>MVLGKPQTDPTLEWFLSHCHIHKYPSKSTLIHQGEKAETLYYIVKGSVAVLIKDEEGKEMILSYLNQGDFIGELGLFEEGQERSAWVRAKTACEVAEISYKKFRQLIQVNPDILMRLSAQMARRLQVTSEKVGNLAFLLVTGRIAQTLLNLAKQPDAMTHPDGMQIKITRQEI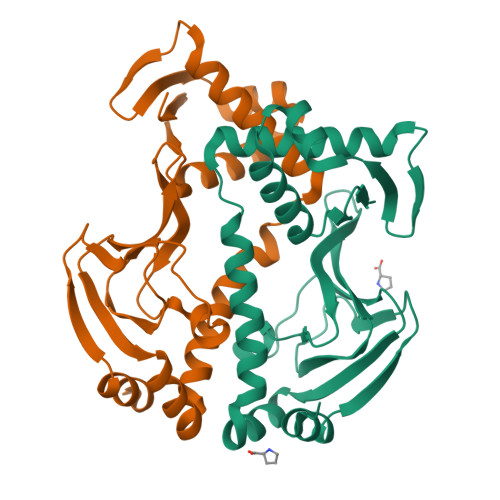GQIVGCSRETVGRILKMLEDQNLISAHGKTIVVYGTR[2x]>[2x]VIEKVQHIQLLQKNVRAQLVDMKRLEVDIDIKIRSCRGSCSRALAREVDLKDYEDQQKQLEQVIAK;>[2x]HQLYIDETVNSNIPTNLRVLRSILENLRSKIQKLESDVSAQMEYCRTPCTVSCNIPVVSGKECEEIIRKGGETSEMYLIQPDSSVKPYRVYCDMNTENGGWTVIQNRQDGSVDFGRKWDPYKQGFGNVATNTDGKNYCGLPGEYWLGNDKISQLTRMGPTELLIEMEDWKGDKVKAHYGGFTVQNEANKYQISVNKYRGTAGNALMDGASQLMGENRTMTIHNGMFFSTYDRDNDGWLTSDPRKQCSKEDGGGWWYNRCHAANPNGRYYWGGQYTWDMAKHGTDDGVVWMNWKGSWYSMRKMSMKIRPFFPQQ;>YEASILTHDSSIRYLQEIYNSNNQKIVNLKEKVAQLEAQCQEPCKDTVQIHDITGKDCQDIANKG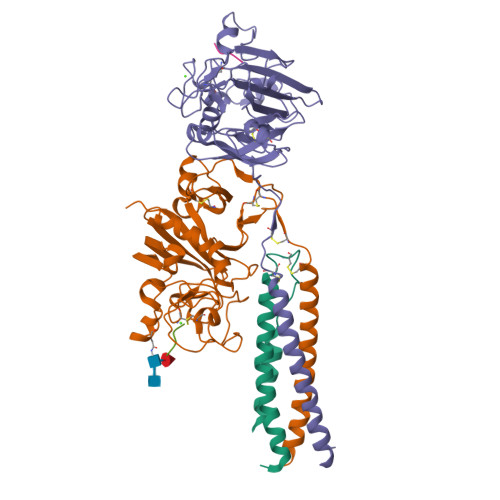AKQSGLYFIKPLKANQQFLVYCEIDGSGNGWTVFQKRLDGSVDFKKNWIQYKEGFGHLSPTGTTEFWLGNEKIHLISTQSAIPYALRVELEDWNGRTSTADYAMFKVGPEADKYRLTYAYFAGGDAGDAFDGFDFGDDPSDKFFTSHNGMQFSTWDNDNDKFEGNCAEQDGSGWWMNKCHAGHLNGVYYQGGTYSKASTPNGYDNGIIWATWKTRWYSMKKTTMKIIPFNRLTIGEGQQHHLGGAK[2x];>[4x]GPRVVE>MVLYFIGLGLYDERDITVKGLEIAK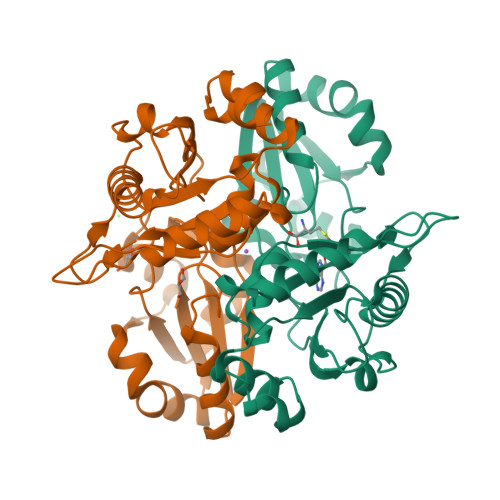KCDYVFAEFYTSLMAGTTLGRIQKLIGKEIRVLSREDVERNFENIVLPLAKENDVAFLTPGDPLVATTHAELRIRAKRAGVESYVIHAPSIYSAVGITGLHIYKFGKSATVAYPEGNWFPTSYYDVIKENAERGLHTLLFLDIKAEKRMYMTANEAMELLLKVEDMKKGGVFTDDTLVVVLARAGSLNPTIRAGYVKDLIREDFGDPPHILIVPGKLHIVEAEYLVEIAGAPREILRVNV[2x]>[4x]MSVGIVYGDQYRQLCCSSPKFGDRYALVMDLINAYKLIPELSRVPP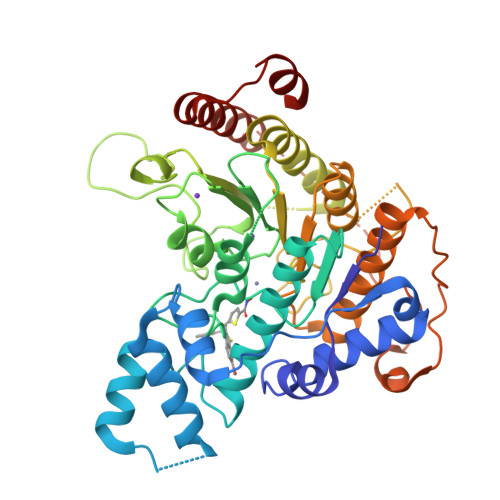LQWDSPSRMYEAVTAFHSTEYVDALKKLQMLHCEEKELTADDELLMDSFSLNYDCPGFPSVFDYSLAAVQGSLAAASALICRHCEVVINWGGGWHHAKRSEASGFCYLNDIVLAIHRLVSSTPPETSPNRQTRVLYVDLDLHHGDGVEEAFWYSPRVVTFSVHHASPGFFPGTGTWNMVDNDKLPIFLNGAGRGRFSAFNLPLEEGINDLDWSNAIGPILDSLNIVIQPSYVVVQCGADCLATDPHRIFRLTNFYPNLNLDSDCDSECSLSGYLYAIKKILSWKVPTLILGGGGYNFPDTARLWTRVTALTIEEVKGKKMTISPEIPEHSYFSRYGPDFELDIDYFPHKSHNKTLDSIQKHHRRILEQLRNYADLNKLIYDYDQVYQLYNLTGM>GSHMGTRDDEYDYLFKVVLIGDSGVGKSNLLSRFTRNEFNLESKSTIGVEFATRSIQVDGKTIKAQIWDTAGLERYRAITSAYYRGAVGALLVYDIAKHLTYENVERWLKELRDHADSNIVIMLVGNKSDLRHLRAVPTDEARAFAEKNGLSFIETSALDSTNVEAAFQTILTEIYRIVSQKQMSDRRENDMSPSNNVVPIHVPPTTENKPKVQCCQNI[4x];>[4x]GMDAALKRSRSEEPAEILPPARDEEEEEEEGMEQGLEEEEEVDPRIQGELEKLNQSTDDINRRETELEDARQKFRSVLVEATVKLDELVKKIGKAVEDSKPYWEARRVARQAQLEAQKATQDFQRATEVLRAAKETIS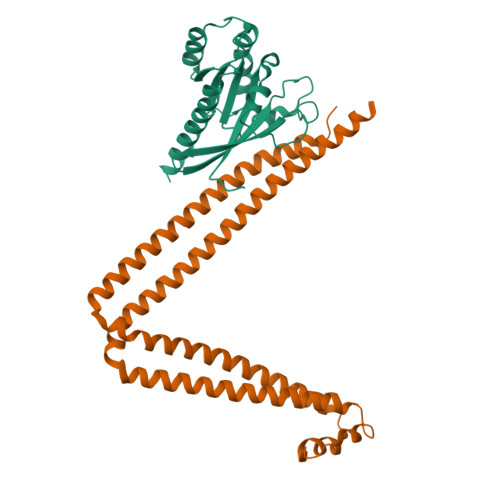LAEQRLLEDDKRQFDSAWQEMLNHATQRVMEAEQTKTRSELVHKETAARYNAAMGRMRQLEKKLKRAINKSKPYFELKAKYYVQLEQLKKTVDDLQAKLTLAKGEYKMALKNLEMISDEIHERRRSSA>MPKRTDIKSILILGAGPIVIGQACEFDYSGAQACKALREEGYRVINVNSNPATIMTDPEMADATYIEPIHWEVVRKIIEKERPDAVLPTMGGQTALNCALELERQGVLEEFGVTMIGATADAIDKAEDRRRFDVAMKKIGLETARSGIAHTMEEALAVAADVGFPCIIRPSFTMGGSGGGIAYNREEFEEICARGLDLSPTKELLIDESLIGWKEYEMEVVRDKNDNCIIVCSIENFDAMGIHTGDSITVAPAQTLTDKEYQIMRNASMAVLREIGVETGGSNVQFAVNPKNGRLIVIEMNPRVSRSSALASKATGFPIAKVAAKLAVGYTLDELMNDITGGRTPASFEPSIDYVVTKIPRFNFEKFAGANDRLTTQMKSVGEVMAIGRTQQESLQKALRGLEVGATGFDPKVSLDDPEALTKIRRELKDAGADRIWYIADAFRAGLSVDGVFNLTNIDRWFLVQIEELVRLEEKVAEVGITGLNADFLRQLKRKGFADARLAKLAGVREAEIRKLRDQYDLHPVYKRVDTCAAEFATDTAYMYSTYEEECEANPSTDREKIMVLGGGPNRIGQGIEFDYCCVHASLALREDGYETIMVNCNPETVSTDYDTSDRLYFEPVTLEDVLEIVRIEKPKGVIVQYGGQTPLKLARALEAAGVPVIGTSPDAIDRAEDRERFQHAVERLKLKQPANATVTAIEMAVEKAKEIGYPLVVRPSYVLGGRAMEIVYDEADLRRYFQTAVSVSNDAPVLLDHFLDDAVEVDVDAICDGEMVLIGGIMEHIEQAGVHSGDSACSLPAYTLSQEIQDVMRQQVQKLAFELQVRGLMNVQFAVKNNEVYLIEVNPRAARTVPFVSKATGVPLAKVAARVMAGKSLAEQGVTKEVIPPYYSVKEVVLPFNKFPGVDPLLGPEMRSTGEVMGVGRTFAEAFAKAQLGSNSTMKKHGRALLSVREGDKERVVDLAAKLLKQGFELDATHGTAIVLGEAGINPRLVNKVHEGRPHIQDRIKNGEYTYIINTTSGRRAIEDSRVI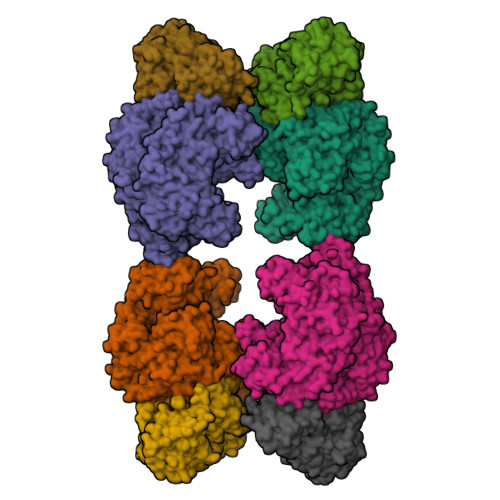RRSALQYKVHYDTTLNGGFATAMALNADATEKVISVQEMHAQIK[4x];>MIKSALLVLEDGTQFHGRAIGATGSAVGEVVFNTSMTGYQEILTDPSYSRQIVTLTYPHIGNVGTNDADEESSQVHAQGLVIRDLPLIASNFRNTEDLSSYLKRHNIVAIADIDTRKLTRLLREKGAQNGCIIAGDNPDAALALEKARAFPGLNGMDLAKEVTTAEAYSWTQGSWTLTGGLPQAKKEDELPFHVVAYDFGAKRNILRMLVDRGCRLTIVPAQTSAEDVLKMNPDGIFLSNGPGDPAPCDYAITAIQKFLETDIPVFGICLGHQLLALASGAKTVKMKFGHHGGNHPVKDVEKNVVMITAQNHGFAVDEATLPANLRVTHKSLFDGTLQGIHRTDKPAFSFQGHPEASPFPHDAAPLFDHFIELIEQYRKTAK[4x]>GSTEVQKNQVLTLEEWQDKWVNGKTAFHQEQGHQLLKKHLDTFLKGKSGLRVFFPLCGKAVEMKWFADRGHSVVGVEISELGIQEFFTEQNLSYSEEPITEIPGTKVFKSSSGNISLYCCSIFDLPRTNIGKFDMIWDRGALV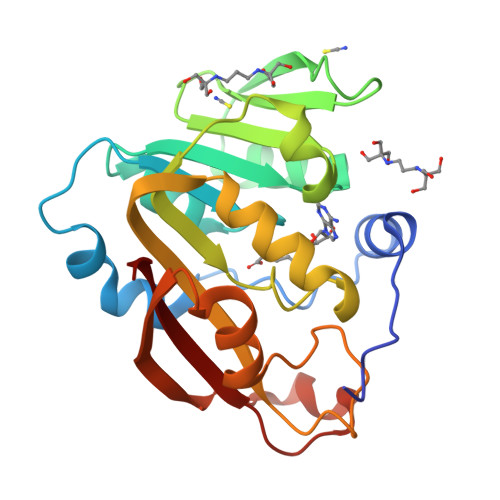AINPGDRKCYADTMFSLLGKKFQYLLCVLSYDPTKHPGPPFYVPHAEIERLFGKICNIRCLEKVDAFEERHKSWGIDCLFEKLYLLTEK[2x]> MASQSSVAVISSAAARGESFPDSKKPIGSVRFQQPLRLSFSYCKSGNMSSRICAMAKPNDAETLSSSVDMSLSPRVQSLKPSKVMVITDLAATLVQSGVPVIRLAAGEPDFDTPKVVAEAGINAIREGFTRYTLNAGITELREAICRKLKEENGLSYAPDQILVSNGAKQSLLQAVLAVCSPGDEVIIPAPYWVSYTEQARLADATPVVIPTKISNNFLLDPKDLESKLTEKSRLLILCSPSNPTGSVYPKSLLEEIARIIAKHP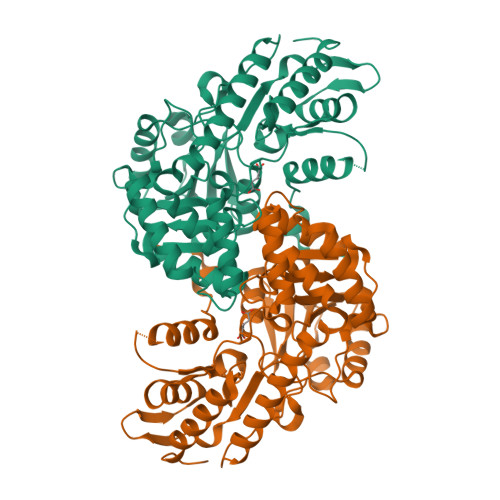RLLVLSDEIYEHIIYAPATHTSFASLPDMYERTLTVNGFSKAFAMTGWRLGYLAGPKHIVAACSKLQGQVSSGASSIAQKAGVAALGLGKAGGETVAEMVKAYRERRDFLVKSLGDIKGVKISEPQGAFYLFIDFSAYYGSEAEGFGLINDSSSLALYFLDKFQVAMVPGDAFGDDSCIRISYATSLDVLQAAVEKIRKALEPLRATVSV> ETKFVQALFDFNPQESGELAFKRGDVITLINKDDPNWWEGQLNNRRGIFPS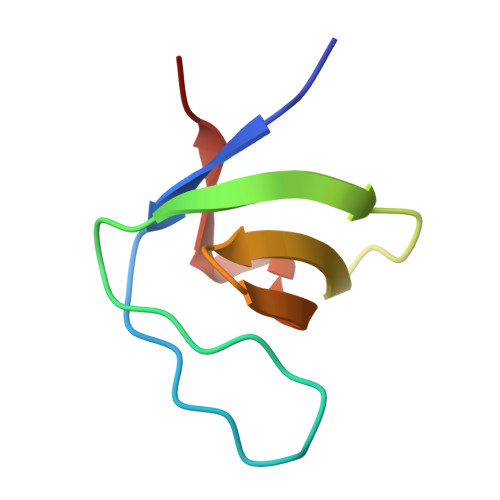NYVCPYNSN>HEHNTIPKGASIEVKVQQLDPVNGNKDVGTVTITESNYGLVFTPDLQGLSEGLHGFHIHENPSCEPKEKEGKLT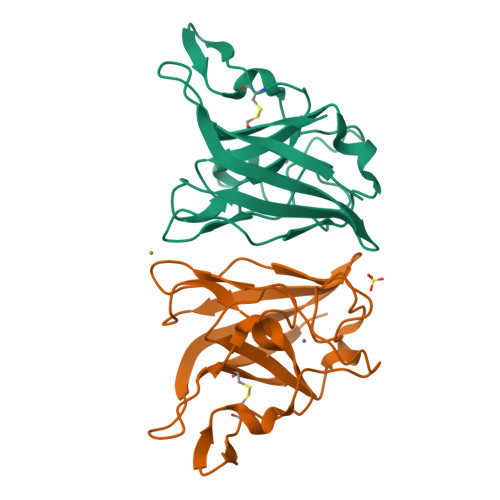AGLGAGGHWDPKGAKQHGYPWQDDAHLGDLPALTVLHDGTATNPVLAPRLKHLDDVRGHSIMIHTGGDNHSDHPAPLGGGGPRMACGVIK[3x]> ISEFARTQ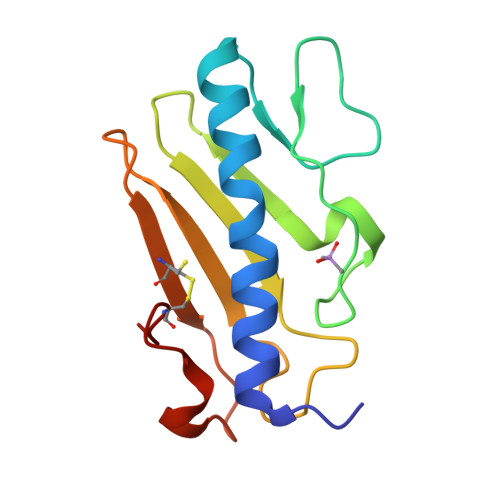VTRAVSEVSALKTAAESAILEGKEIVSSATPKDTQYDIGFTESTLLDGSGKSQIQVTDNKDGTVELVATLGKSSGSAIKGAVITVSRKNDGVWNCKITKTPTAWKPNYAPANCPKS>MASPQLQMALDGFKMMGEKMAQAGGDVKAMRAVMEEMATFPSAGETKCTPVNAGGVPAEWIAAPGAADDRVILYLHGGGYVMGSITTHRETIARLSKASGARALALDYRLAPEYPFPAAVDDATAAYRWLLSQDIKPSRIVVAGDSAGGGLVLATLVALRDAKVPLPAAGVCISPWADMEGTGASMTTRAKADPVVQKEMLVNMGKTYLGGKDAKSPLAAPLHADFRGLPPLFIQVGDAETLLDDSTRVAEKAKMAGVKVDLEIWPEMPHVWHLFAP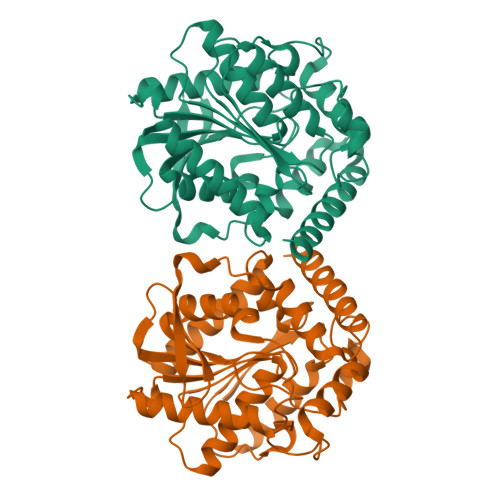FLPEGQQAIDKIGQYVKQRTAHHHHHH[4x]> GGGG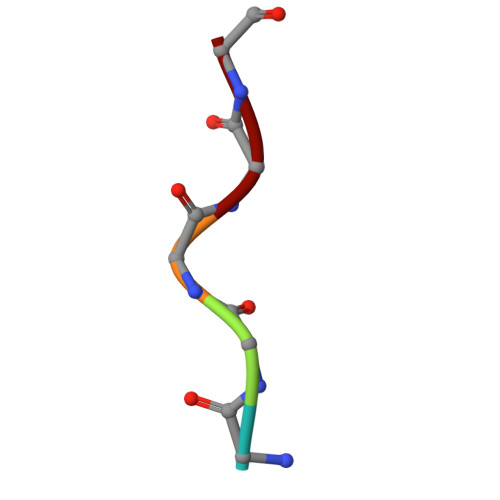G>SMGPGVWDPNWDRREPLSLINVRKRNVESGEEELASKLDHYKAKATRHIFLIRHSQYHVDGSLEKDRTLTPLGREQAELTGLRLASLGLKFNKIVHSSMTRAIETTDIISRHLPGVCKVSTDLLREGAPIEPDPPVSHWKPEAVQYYEDGARIEAAFRNYIHRADARQEEDSYEIFICHANVI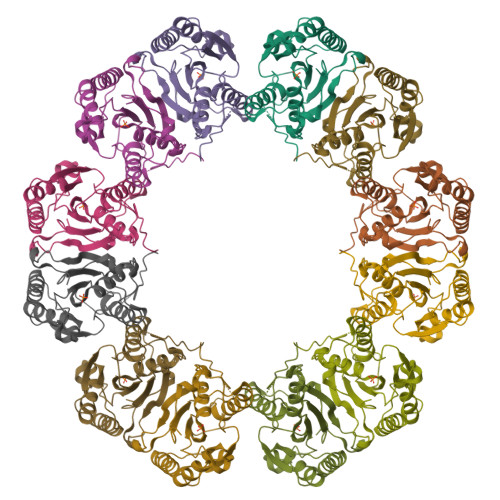RYIVCRALQFPPEGWLRLSLNNGSITHLVIRPNGRVALRTLGDTGFMPPDKITRS[3x]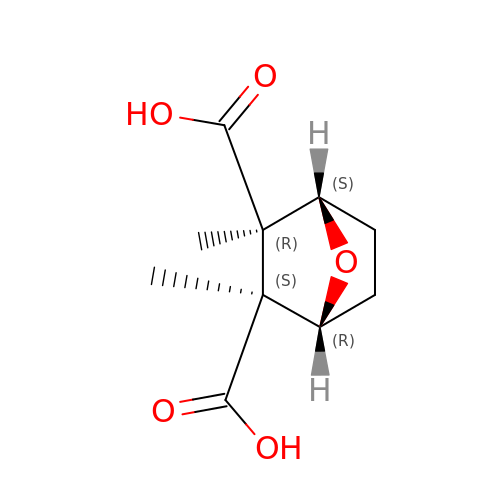(1R,2S,3R,4S)-2,3-dimethyl-7-oxabicyclo[2.2.1]heptane-2,3-dicarboxylic acid | C10 H14 O5 | NMTNUQBORQILRK-XCVPVQRUSA-N> AE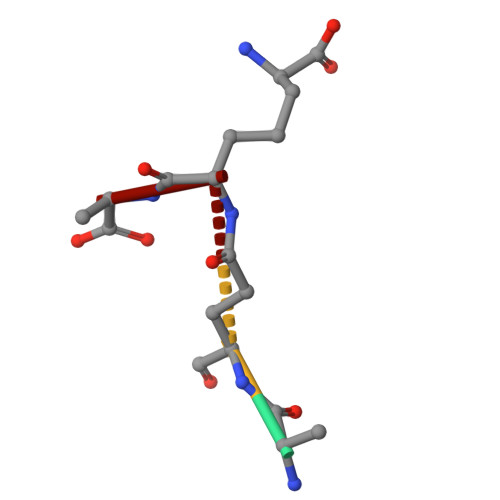KA>MAHPDEELLPPAPKYNTKTSEQEPGDWKQPTESLTLNRLCEIAQAWASMTWEDIDDKQLRALLTLSAVLVRKHSKSQLSALCENHVRREALAQDQASIVLEVYQKLHSDKGGKFEAALWQHWDRGSLTLFIHAALRA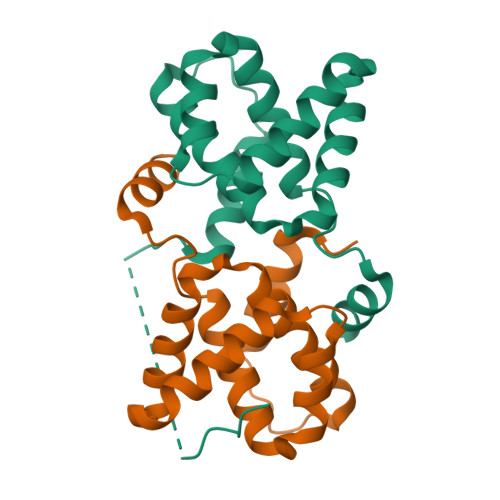GTTIPCESSAIVVASIMSLLSNSQNDSLEHHHHHH[2x]Plants sense abscisic acid (ABA) using chemical-induced dimerization (CID) modules, including the receptor PYR1 and HAB1, a phosphatase inhibited by ligand-activated PYR1. ABA binds to PYL receptors and stabilizes activated conformers that bind and inhibit type 2C protein phosphatases (PP2Cs), which prevents the PP2Cs from dephosphorylating and inactivating their downstream stress-activated SnRK2 kinase targets. PYR1’s phosphatase partner acts analogously to a co-receptor, boosting apparent ligand-binding affinity up to ~100-fold. To expand the PYR1 system, we designed an orthogonal ‘*’ module, which harbors a dimer interface salt bridge; X-ray crystallographic, biochemical and in vivo analyses confirm its orthogonality.

To determine if the orthogonalized module’s ligand recognition could be reprogrammed, we ‘grafted’ the T162D/V393R mutations onto the previously engineered receptor PYR1MANDI and HAB1. The mutant receptor responded to mandi in Y2H assays but with ~100-fold reduced sensitivity compared to the PYR1MANDI/HAB1 interaction. We, therefore, mutagenized M158, F159 and A160 in the C-terminal α-helix and identified mutations in these residues that increase module sensitivity using Y2H-based selections, yielding the nonuple mutant PYR1*MANDI (PYR1Y58H;K59R;V81I;F108A; S122G;M158I;F159V;A160V;T162D). Additional mutagenesis of HAB1V393R,R505A,D204A followed by positive selections led to a catalytically inactive, pentuple mutant that we call HAB1* (HAB1R199A;D204A;S322D;V393R;R505A). The final PYR1*MANDI/HAB1* CID module responds to low nM mandi concentrations in Y2H assays, selectively binds to HAB1* and does not strongly regulate WT HAB1’s phosphatase activity, which together indicate sensitive and orthogonal function of the final PYR1*MANDI/HAB1* CID module. The extensive mutagenesis required to engineer high-sensitivity mandi responsiveness prompted us to obtain an X-ray crystal structure of a PYR1*MANDI/mandi/HAB1* ternary complex, which we solved at 2.4-Å resolution. As expected, the ligand–receptor contacts mirror those of the original PYR1MANDI; the module is nearly superimposable with WT modules (CA RMSD of 1.7 Å); and the electron density map confirms the absence of metal ions in HAB1’s catalytic site. The structure reveals the consequences of the orthogonalizing T162D/V393R mutations, which form a salt bridge positioned 2.7 Å from one another. Thus, our mutational pipeline created an orthogonal signaling module by introducing a salt bridge in the PYR1*MANDI/HAB1* binding interface with minimal changes to the module’s global structure.

> MPSELTPEERSELKNSIAEFHTYQLDPGSCSSLHAQRIHAPPELVWSIVRRFDKPQTHRHFIKSCSVEQNFEMRVGCTRDIIVISGLPANTSTERLDILDDERRVTGASIIGGEHRLTNYKGVTTVHRFEKENRIWTVVLESYVVDMPEGNSEDDTRIVVDDVVKLNLQKLATVAEAMARN;> RSVYELDCIPLWGTVSIQGNASEMEAAFAVSPHFLKLPIKMLMGDHEGMSPSLTHLTGHFFGVYDGHGGHKVADYCRDRLHFALAEEIERIKDELCKRNTGEGRQVQWDKVFTSCFLTVDGEIEGKIGRAVVGSSDKVLEAVADETVGSTAVVALVCSSHIVVSNCGDSRAVLFRGKEAMPLSVDHKPDREDEYARIENAGGKVIQWQGARVFGRLAMSRSIGDRYLKPYVIPEPEVTFMPRSREDECLILASDGLWDVMNNQEVCEIARRRILMWHKKNGAPPLAERGKGIDPACQAAADYLSMLALQKGSKDNISIIVIDLKAQRKFKTAT> MDWRHKAVCRDEDPELFFPVGNSGPALAQI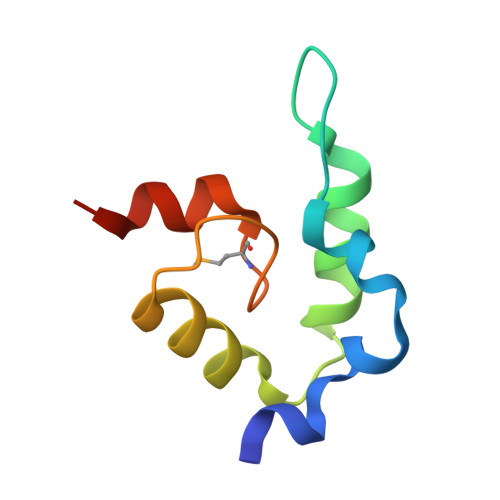ADAKLVCNRCPVTTECLSWALNTGQDSGVWGGMSEDERRALKRRNA> MSLSNKLTLDKLDVKGKRVVMRVDFNVPMKNNQITNNQMIKAAVPSIKFCLDNGAKSVVLMSHLGRPDGVPMPDKYSLEPVAVELKSLLGKDVLFLKDCVGPEVEKACANPAAGSVILLENLRFHVEEEGKGKDASGNKVKAEPAKIEAFRASLSKLGDVYVNDAFGTAHRAHSSMVGVNLPQKAGGFLMKKELNYFAKALESPERPFLAILGGAKVADKIQLINNMLDKVNEMIIGGGMAFTFLKVLNNMEIGTSLFDEEGAKIVKDLMSKAEKNGVKITLPVDFVTADKFDENAKTGQATVASGIPAGWMGLDCGPESSKKYAEAVTRAKQIVWNGPVGVFEWEAFARGTKALMDEVVKATSRGCITIIGGGDTATCCAKWNTEDKVSHVSTGGGASLELLEGKVLPGVDALSNI

Phosphoglycerate kinase 1 (PGK1) is an ubiquitous enzyme expressed in all somatic cells that plays a central role in glycolysis where it provides energy in form of ATP through the reversible phosphotransfer reaction from 1,3-bisphosphoglycerate (1,3-BPG) to MgADP in order to produce 3-phosphoglycerate (3-PG) and MgATP in the presence of free magnesium. PGK1 is a monomeric enzyme of 417 amino acids formed by two distinct α-helical domains of equal size, the N- and C-terminal domains connected by a hinge region. The N-terminal domain binds 3-PG or 1,3-BPG while the C-terminal domain binds MgADP or MgATP. Two different crystallographic conformations of PGK1 have been already identified: the partially closed conformation, able to bind substrates, and the closed conformation, the catalytically competent state.

The residue R38 is placed in the N-terminal 3-PG binding domain and is a residue important for the substrate binding and its correct positioning towards the co-substrate MgADP. Moreover, together with residues K215 and K219, R38 is critical for the charge balancing of the transition state, directly interacting with the transferring phosphate group in the closed conformation of PGK1. The crystal structure of R38M contains ADP but does not contain 3-PG, in line with the role of R38. The absence of the 3-PG ligand could account even for the variant reluctance to crystallize in the closed form since the binding of both substrates is required for the stabilization of this conformation. Taken together these observations justify the dramatic effect of R38M mutation on kinetic parameters. All the variants display a reduced catalytic efficiency, particularly evident for the variant R38M, that shows a decrease of eight order of magnitude of the kcat/KM value, mainly due to a dramatic decrease of the turnover number. As shown in the structure, R38 is located in the 3-PG binding site and interacts electrostatically with the carboxyl group of 3-PG, hence it is critical for the positioning of the substrate in the catalytic site and for the stabilization of the transition state. Accordingly, the substitution of the R38 implies a dramatic decrease of the kcat and an increase of Km. In this regard, R38, replaced with a methionine in the variant R38M, is placed in a critical position.NEOPTERIN | C9 H11 N5 O4 | 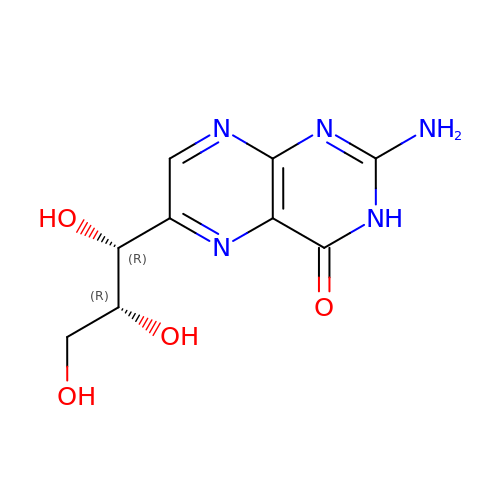BMQYVXCPAOLZOK-INEUFUBQSA-N> MEDEIRK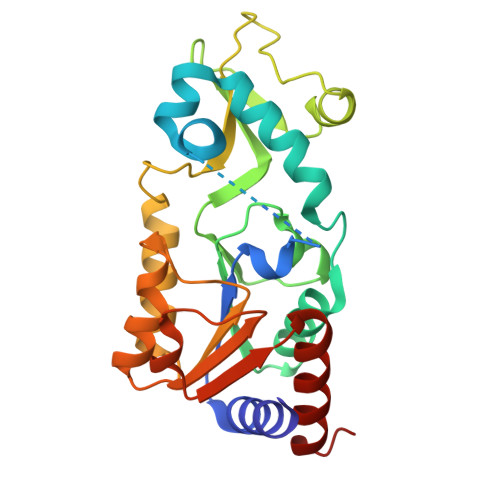AAEILAKSKHAVVFTGAGISAESGIPTFRGEDGLWRKYDPEEVASISGFKRNPRAFWEFSMEMKDKLFAEPNPAHYAIAELERMGIVKAVITQNIDMLHQRAGSRRVLELHGSMDKLDCLDCHETYDWSEFVEDFNKGEIPRCRKCGSYYVKPRVVLFGEPLPQRTLFEAIEEAKHCDAFMVVGSSLVVYPAAELPYIAKKAGAKMIIVNAEPTMADPIFDVKIIGKAGEVLPKIVEEVKRLRSEK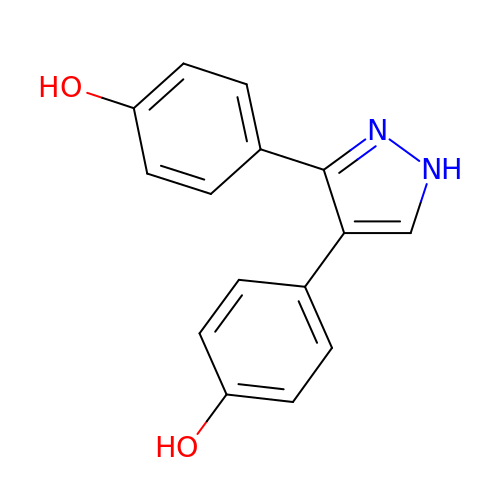4,4'-(1H-pyrazole-3,4-diyl)diphenol | C15 H12 N2 O2 | FHGTUVGVZRNUDB-UHFFFAOYSA-N> MPVTINNFNYNDPIDNNNIIMMEPPFARGTGRYYKAFKITDRIWIIPERYTFGYKPEDFNKSSGIFNRDVCEYYDPDYLNTNDKKNIFLQTMIKLFNRIKSKPLGEKLLEMIINGIPYLGDRRVPLEEFNTNIASVTVNKLISNPGEVERKKGIFANLIIFGPGPVLNENETIDIGIQNHFASREGFGGIMQMKFCPEYVSVFNNVQENKGASIFNRRGYFSDPALILMHQLIYVLHGLYGIKVDDLPIVPNEKKFFMQSTDAIQAEELYTFGGQDPSIITPSTDKSIYDKVLQNFRGIVDRLNKVLVCISDPNININIYKNKFKDKYKFVEDSEGKYSIDVESFDKLYKSLMFGFTETNIAENYKIKTRASYFSDSLPPVKIKNLLDNEIYTIEEGFNISDKDMEKEYRGQNKAINKQAYEEISKEHLAVYKIQMCKSVKAPGICIDVDNEDLFFIADKNSFSDDLSKNERIEYNTQSNYIENDFPINELILDTDLISKIELPSENTESLTDFNVDVPVYEKQPAIKKIFTDENTIFQYLYSQTFPLDIRDISLTSSFDDALLFSNKVYSFFSMDYIKTANKVVEAGLFAGWVKQIVNDFVIEANKSNTMDKIADISLIVPYIGLALNVGNETAKGNFENAFEIAGASILLEFIPELLIPVVGAFLLESYIDNKNKIIKTIDNALTKRNEKWSDMYGLIVAQWLSTVNTQFYTIKEGMYKALNYQAQALEEIIKYRYNIYSEKEKSNINIDFNDINSKLNEGINQAIDNINNFINGCSVSYLMKKMIPLAVEKLLDFDNTLKKNLLNYIDENKLYLIGSAEYEKSKVNKYLKTIMPFDLSIYTNDTILIEMFNKYNSEILNNIILNLRYKDNNLIDLSGYGAKVEVYDGVELNDKNQFKLTSSANSKIRVTQNQNIIFNSVFLDFSVSFWIRIPKYKNDGIQNYIHNEYTIINCMKNNSGWKISIRGNRIIWTLIDINGKTKSVFFEYNIREDISEYINRWFFVTITNNLNNAKIYINGKLESNTDIKDIREVIANGEIIFKLDGDIDRTQFIWMKYFSIFNTELSQSNIEERYKIQSYSEYLKDFWGNPLMYNKEYYMFNAGNKNSYIKLKKDSPVGEILTRSKYNQNSKYINYRDLYIGEKFIIRRKSNSQSINDDIVRKEDYIYLDFFNLNQEWRVYTYKYFKKEEMKLFLAPIYDSDEFYNTIQIKEYDEQPTYSCQLLFKKDEESTDEIGLIGIHRFYESGIVFEEYKDYFCISKWYLKEVKRKPYNLKLGCNWQFIPKDEGWTELEVLFQGPLEHHHHHH

The botulinum neurotoxins (BoNT) are potent bacterial toxins produced mainly by toxigenic Clostridium botulinum species. The holotoxins are expressed as single-chain proteins that need to be proteolytically activated into a functional di-chain form, which consists of a ~50 kDa light chain (LC) linked by a single disulphide bond to the ~100 kDa heavy chain (HC). Although they all share a common modular architecture based on the three functional domains necessary for their activity, namely the binding (HC) and translocation domains (HN), which form HC and the catalytic (LC) domain, they present distinctive properties. Serotypes A, B and E are the main BoNT associated with human botulism. These neurotoxins specifically target presynaptic motoneurons via a dual-receptor binding mechanism, which involves membrane-anchored gangliosides and a protein receptor.

Complete movies were collected on a Titan Krios microscope, resulting in EM maps at 3.6 and 3.7Å average resolution for BoNT/B and BoNT/E, respectively, although local resolution varied significantly. Here, BoNT/B also presents a linear arrangement of its three domains, whereas the BoNT/E map shows it retained its more compact domain organisation, thus alleviating reservation that this singular domain organisation among BoNTs may have been experimental artefacts. Our structures are of inactive variants of the toxins presenting dual mutations at the catalytic site (BoNT/B1 E231Q/H234Y and BoNT/E1 E213Q/H216Y). A similar set of mutations (i.e., HQxxY) in BoNT/A was previously shown to prevent binding of the catalytic Zn2+ ion, which is also not visible in either of the two maps presented here. In the cryo-EM map of BoNT/B, the belt is well-ordered except for a small surface-exposed α-helix (residues 487–495), whereas in BoNT/E, a section could not be modelled due to the lack of map for residues 499–515, which forms a random coil in the crystal structure. For BoNT/B, the lack of density in some areas, particularly the HCC subdomain, suggests that the preferred particle orientation observed in the angular distribution map is the main reason affecting map quality and resolution, although local dynamism of the domain cannot be excluded. Since HC/B has been well defined by X-ray crystallography, it was fully included in the deposited coordinates associated with the map. Although the crystal structures of BoNT/B and BoNT/E were used to produce the cryo-EM models some differences were observed when comparing the output from both methods, with direct superposition showing root mean square deviations of 1.9 Å (over 1218 paired residues) and 2.0 Å (over 1197 paired residues) for types B and E, respectively. For example, overall superposition with BoNT/B results in a nearly perfect overlap of the translocation domains, whilst the core secondary structure of LC appears shifted by approximately 1.5 Å, with some of the larger loops deviating more significantly.> EEGLDFPEYDGVDRVVNVNAKNYKNVFKKYEVLALLYHEPPEDDKASQRQFEMDELILELAAQVLEDKGVGFGMVDSEKDAAVAKKLGLTEEDSVYVFKGDEVIEYDGEFSADTLVEFLLDVLEDPVELIEGERELQAFENIEDDNKLIGYFKNKDSEHYKAYEDAAEEFHPYIPFFATFDSKVAKKLTLKLNEIDFYEAFMEEPVTIPDKPNSEEEIVSFVEAHKRSTLRKLKPESMYETWEDDLDGIHIVAFAEETDPDGYEFLETLKAVAQDNTDNPDLSIIWIDPDDFPLLVPYWEKTFNIDLSAPQIGVVNVTDADSVWMEMDDEEDLPSAEELEDWLEDVLEGEINTEDDDEEDD

Calsequestrin (Casq) is considered to be the major Ca2+-storage/buffer protein within the sarcoplasmic reticulum (SR) of both cardiac and skeletal muscle, where it resides as either its cardiac (Casq2) or skeletal (Casq1) isoform. Casq binds Ca2+ with a capacity roughly equivalent to a half of its total negative charge and an overall dissociation constant of ~1 mM. When studied in solution, Casq polymerizes as free Ca2+ concentrations increase and depolymerizes as Ca2+ concentrations decrease. We also showed that both glycosylation and phosphorylation alter the physical characteristics of Casq substantially, including its oligomerization and Ca2+-binding capacity.

To investigate any structural significance/role of glycans or structural change due to the presence of glycans, the crystal structures for both native and recombinant bovine Casq1, which correspond to the glycosylated and nonglycosylated form, respectively, were determined under the same condition. Calsequestrin crystallized in two forms: the low-Ca2+ forms of native and recombinant bovine Casq1 crystallized in the absence of added Ca2+ in the crystallization buffer; the high-Ca2+ forms crystallized in the presence of 2.5 mM Ca2+ (17× molar excess of Ca2+ added to solution). Low-Ca2+ native bovine Casq1 crystallized in the P1 space group and contained four molecules in the unit cell; the resolution of its diffraction data was 2.74 Å, whereas low-Ca2+ recombinant bovine Casq1 crystallized in the C2221 space group and contained one molecule in the asymmetric unit, with a resolution of 1.88 Å. The lattice packing for both low-Ca2+ native and recombinant established a typical weakly-interacting linear polymer with D2 symmetry, a pattern also found in previous Casq structures. Each monomer in the low-Ca2+ structures of both native and recombinant Casq1 contained five Ca2+ ions, while the three monomers in the high-Ca2+ asymmetric units contained a total of 38 Ca2+ ions. Superposition of low-Ca2+ recombinant Casq1 onto the four low-Ca2+ native monomers in the P1 unit cell had an average r.m.s.d of 0.40 Å.> EGS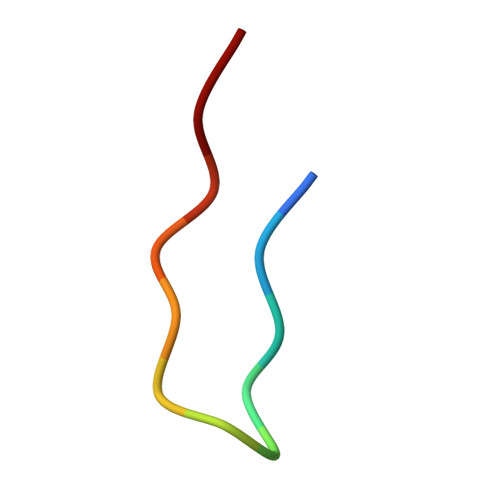ITQGTPLKY> APS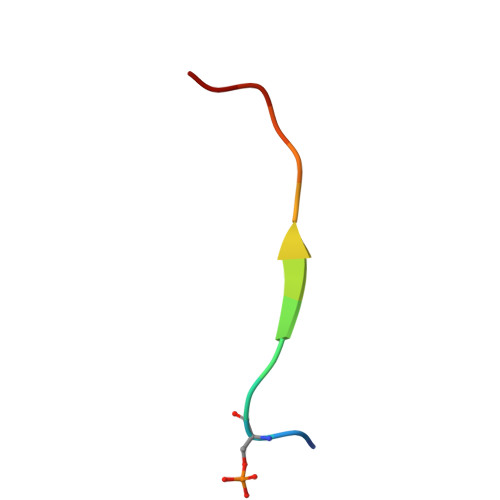TGGVMKPHRYR> MGSSHHHHHHSSGLVPRGSHSEQKLISEEDLSMASISKDFTNLLNTLIDGQIGAASRQTEWFNMSPDERTDYIKQVDERLQEMQQSTLSVLAAQHFQMQDNPVSVGDQLQTLQKRRQQMTDVPGTPAINAYKQQLDRDILLYRRQQTAMTHFDSTWRKVLVMLGPDDSKPLNATTLRENAVDKQAKLDTEIKRLEQQLTIQVADSTFSQKYVTLFSELQAYKDVNARYNALLKASATEEAAALGALTKVPQASDDLPVNISLLMMEERPGYIRMNVALVNASTDGRFKDFFLENGRLVVLTDGVLNFSFGTAARSLAWQQQYRLKSEPPSFRSPTYTPIRSVLVKTEFVEKYFANYLVSESTLRGGFKAQLLGNGRKMLLTSVDRKVPNQIGIQVSGQAPNTTITREVPLASALSDLINQNADIASFRTIGLEGFRQSSYHPDRDGLFVNIHELERSVGFAGRQYLLEMPQDNDYLSATPFGVMSVDGDKVSSSHLSKAQTDTLYQYNAAFFEKLEQLRSGGMKASRLFEGSIERTAFVQQLVRLLERNHITPAGVLAPEYPRDNMRDIKGNNLNKVLWEQAFAASVWRSRDNDPLLFRLATRLVKNPAVVKVLQNGYVQSDIAQARELLAPLYEQWRTRAVEAETQRVASANAAQHPSNPKVHVFDQAEVERSLDDKLLILLLTGPQSLEGTDVQLRPMVEAALLSNEGRSLRKQILFHALRPVADSFSKAAAPVNPHAELGVGKIMINNRLNQPDPYLILNTSSEEQAYRDGSYLIKDDKYRSYNQFRPDFKNDATRYMNDLDTPFVGGISGTTQTVSNVLTELFGGALSVKQYWQFQMANAAFMIRNGYHSFFETFYVAARYEPEGADSIGKEMLQMFDKYRVEGSKKALQGKLYDGVMARVLPIINQGLSAADEFHPPRFTRIGPRPALLGQAVKDLELKAGLTSVGDGFEPRQGSADIHQFVTDPVLFAKTHTVSAEALVRSGRLPAEGSAQLVKVGSGLYELEYTEQSANDISSSSIPAYFLGYNGPNQANAVPAYVDIPKRTIAGNFLFTGTLSGGSLVVTSLDANTFRVYHDGRVNSSLLYDNVVMAVDYKDYQIAGTAEGL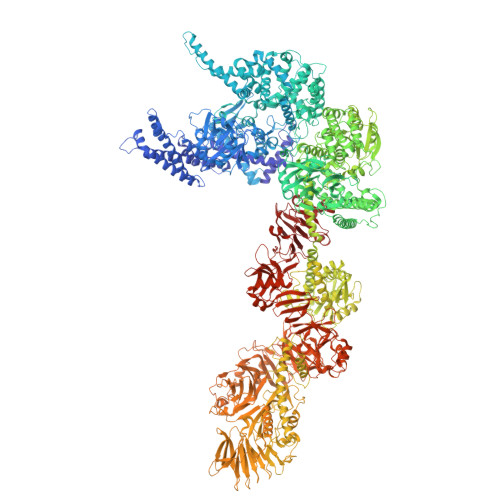AAAYMQYVNHEWQLVLQRQEYQRDGQMLRLRLRDDEEPLSIQVADSQVVERNQAQFVAYREQIHQQLKKVATQFEVSISGVSDGVYTEGEFSPDHPAIAAWAKLCAEVYDRINADTKQLVDKRNKLYENRRNTIRRDLINQQIKQLNITLEYYKAQYDTVLREAGFVEQSWLWQQIKAKNGSAAVVRIDDTAIQGGGKQRTDSVGERYAISEAYQRGARGTGFSDGLRNFREIEIPGVDDKMSALEMKRLFLEGKLTSEQQGALSGRITETSRAEYIDKVLRQTAVFSEDFHDAGSVFDRLVPQDFYLSLVGDRSGGRCYPLVRAMTVALASGGEAGINSLVQKLFFASADPQAGSSTLLRNSLIKLHSNVEAVQASTELGQFGLSEVVSRLAATTGTSMFALNTQNHSMMVGSTVTTEGRRYYFYDPNVGIFAFDNTKSLSRAMEQHLVGRRLAVHYGSFGSKSAPAFNLIEIDTGKMAEVPVGNGLNVADLTRFEELSSVIGQRRQVEQVMSAQERITEDLQLSTALQAFDAEQWGARFEAASTRLAQEHQLDSRWLPIIATTEEQGEGRYRVQFINRDQPEQTRWLDTDDSTFVEFRRFVDEHMSVLNEHFTLESGRMRPRGGVGEAAPVDGLNAGFAVQALIQWFSDKNRHDAANGMASPDLATALKVHSYLNFVQMVHGGVQDVIKVTALVRTALRGEVVAAQTSFKEFALSLGHTVNEGVGVLFGGAMIGLDAYELAHAENDVQKAVFGTQLAFDSASFVTGAAGIGAGLVGASTAGAVLGGAGVILGGLAVGFTALAQAFGAVAEDAKAVGRYFDTVDKAYKGNGYRYDNEKQVLVPLAGAVIKTLDLSKNQIDFDSQYIYRTHSGSTGSGKINYFFWVGDFPRMVHDRGQAIEVRSGIGYKDVSRPLEHGDSNVVILPGTPKSYISYEYMLLPGATTRHDAGFDVIRRLEEDKRFDYDFYIFPGEETIRRIHHEYVDTPIEVVLDQRNRQLVAPELPKELHGFLCYEIKGAGGEYLIGLNEGAKVNLTSDVASTWIIDSSQLASDSISVSKDQLLVGEKGKEVVVKLYLAQNSQVLVVNGKGEVRKVDFTSLTAQVISEDASKWQVPGQQIEQHLSDLAKAHQLHGQYVVVENYRHQGRDVGRAFYDVTKDRMLFTDTTNEQAKRAQLGAVMGDYAYFYDADNAVAWRVDIATGQVDAQFEPWFNQNAGHISRFWQEGDVVYLARRYRLKEREAELGYRIIGDRMELVSAVGDDALLQLSARIGRHGDELEAILQGYRSNSTQRGTLMYTLGARLIQPTSAALVTVFGVDAAGVPHRYWIRTSDGTLIKPNLAPPADQTLHFEAHEQTRSAWQIPADLVLAGSMPLLGGKEVFFFYSKEQKTLFRQEGPGQEVLDANQPSALRVTTPALTNVINLNGHLVVVTEDGRVARLDALGQLSYAAVNEHWLKGRIHWWQDLTSVTDGRATLAVFGVKDTDGKSLLPVWYHNGQVVVASAALQDKHPQFLGFEVDGSSARLFEPASGKLYRQPAMTADALAAAFGTDEVLEASAQLPAANELEPELHLKAAEQVDAGLRLTTVKGEILLRTHDGKLQLVAVDKDWQQDNLVRLSQALAEVAGQWRVKGVLTLQGDDTQGWFDVGSGQVFSIGGIPATDNLRFIGIAVGKKGAYVYNPTDQMLYQVKESGAQKLNHYADVERIGSSLLLQDGGKGDLSPMLIAGVDSVVLHGGAGSDTYRLSQTMWSYYRTVVIDNDDPNQVLDRLIILAVDAEKIFVSRHEDDLMLTDSVNGTVLVIRKVFGSQAVTHRHLQIDLEGSSSVISVDHLVKGFTRLGTANIGLFELPWAIELDYKDDDDK> WE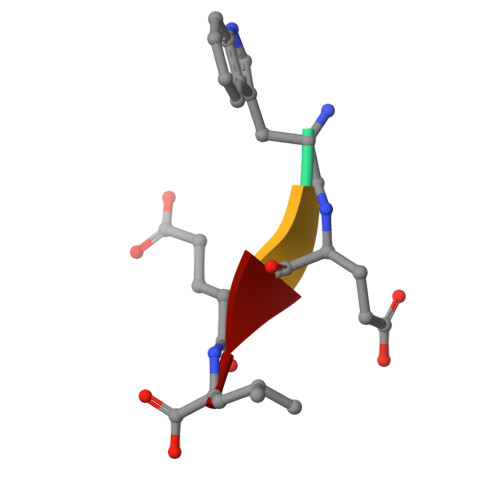EL>[2x]MPEVVFGSVTD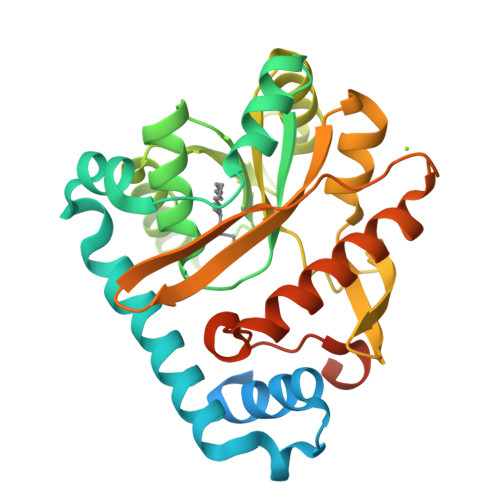LGYAAGWRLVRAMPEAMAQGVFGAGARYAARNGGPEQLRRNLARVVGKPPADVPDDLIRASLASYARYWREAFRLPAMDHGRLGEQLDVIDIDHLWSALDAGRGAVLALPHSGNWDMAGVWLVQNYGPFTTVAERLKPESLYRRFVEYRESLGFEVLPLTGGERPPFEVLAERLTDNRPICLMAERDLTRSGVQVDFFGEATRMPAGPAKLAIETGAALFPVHCWFEGDGWGMRVYPELDTSSGDVTAITQALADRFAANIATYPADWHMLQPQWIADLSDERRARLGTSRHHHHHH>[4x]MKDGMRVGERFTHDFV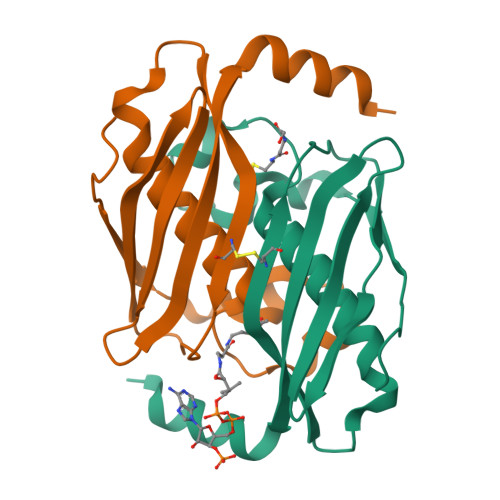VPPHKTVRHLYPESPEFAEFPEVFASGFMVGLMEWACVRAMAPYLEPGEGSLGTAICVTHTAATPPGLTVTVTAELRSVEGRRLSWRVSAHDGVDEIGSGTHERAVIHLEKFNAKVRQKTPAG> TSDSTAPSALIDGPQTGFTMTNDGARTEPDEQDAVYDIMRATGNDWAAAIPDVCRGRWHGIECMPDQDNVYHVVSLSFGALSDDTAFPTCDPQRSYVSESLTRLKHLKALFFYRCLGRAPQRIPAFLGRLGSSLQTLVLRENGFLGPIPDELGNLTNLKVLDLHK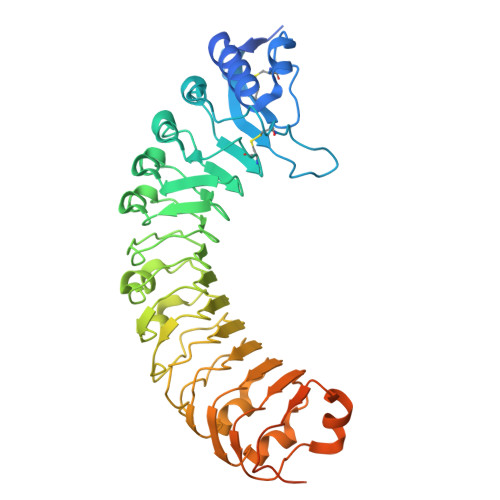NHLNGSIPLSFNRFSGLRSLDLSGNRLTGSIPGFVLPALSVLDLNQNLLTGPVPPTLTSCGSLIKIDLSRNRVTGPIPESINRLNQLVLLDLSYNRLSGPFPSSLQGLNSLQALMLKGNTKFSTTIPENAFKGLKNLMILVLSNTNIQGSIPKSLTRLNSLRVLHLEGNNLTGEIPLEFRDVKHLSELRLNDNSLTGPVPFERDTVWRMRRKLRLYNNAGLCVNRDSDLDDAFGSKSGSTVRLCDAETSRPAPSGTVQHLSREEDGAL> MQDCGLPPDVPNAQPALEGRTSFPEDTVITYKCEESFVK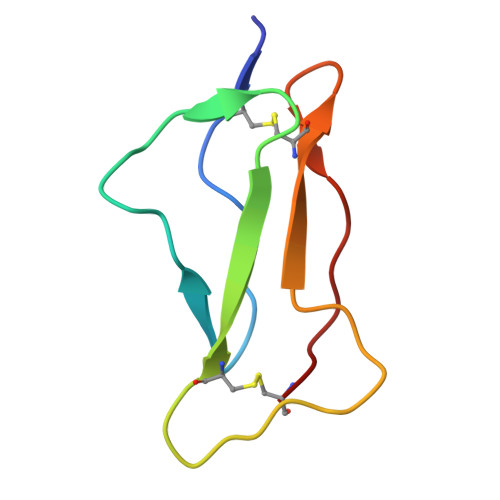IPGEKDSVICLKGSQWSDIEEFC>GPMGTDWPVYHRIDGPIVMIGFGSIGRGTLPLIERHFAFDRSKLVVIDPSDEARKLAEARGVRFIQQAVTRDNYRELLVPLLTAGPGQGFCVNLSVDTSSLDIMELARENGALYIDTVVEPWLGFYFDPDLKPEARSFYALRETVLAARRNKPGGTTAVSCCGANPGMVSWFVKQALVNLAADLGVTGEEPTTREEWARLAMDLGVKGIHIAERDTQRASFPKPFDVFVNTWSVEGFVSEGLQPAELGWGTFERWMPDNARGHDSGCGAGIYLLQPGANTRVRSWTPTAMAQYGFLVTHNESISIADFLTVRDAAGQAVYRPTCHYAYHPCNDAVLSLHEMFGSGKRQSDWRILDETEIVDGIDELGVLLYGHGKNAYWYGSQLSIEETRRIAPDQNATGLQVSSAVLAGMVWALENPNAGIVEADDLDFRRCLEVQTPYLGPVVGVYTDWTPLAGRPGL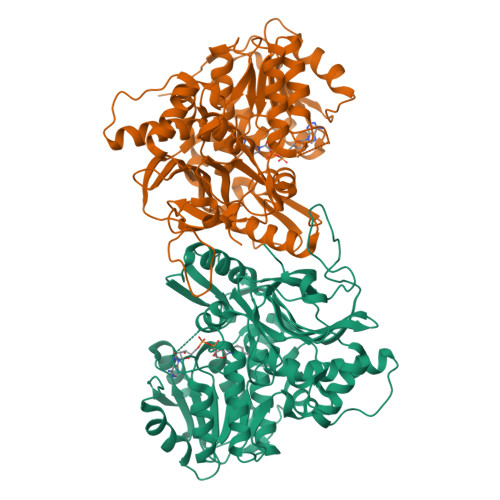FPEDIDTSDPWQFRNVLVRD[2x]> ADTIVAVELDTYPNTDIGDPSYPHIGIDIKSVRSKKTAKWNMQNGKVGTAHIIYNSVGKRLSAVVSYPNGDSATVSYDVDLDNVLPEWVRVGLSASTGLYKETNTILSWSFTSKLKSNSTHETNALHFVFNQFSKDQKDLILQGDATTGTDGNLELTRVSSNGSPQGSSVGRALFYAPVHIWESSAVVASFDATFTFLIKSSDSHPADGIAFFISNIDSSIPSGSTGRLLGLF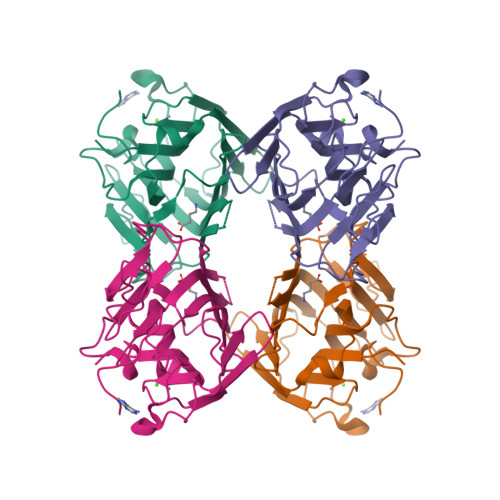PDAN>MSRSGVAVADESLTAFNDLKLGKKYKFILFGLNDAKTEIVVKETSTDPSYDAFLEKLPENDCLYAIYDFEYEINGNEGKRSKIVFFTWSPDTAPVRSKMVYASSKDALRRALNGVSTDVQGTDFSEVSYDSVL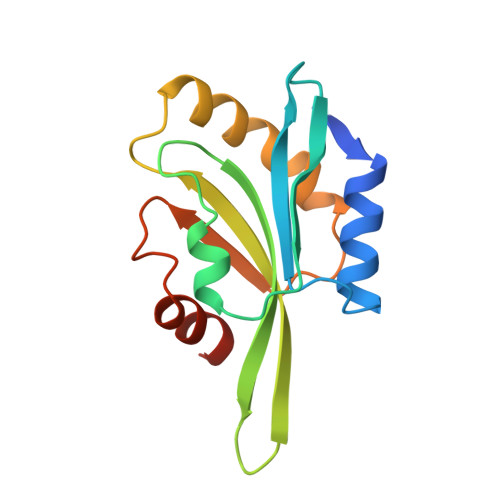ERVSRGAGSH[2x]>MAHHHHHHMPSERTFI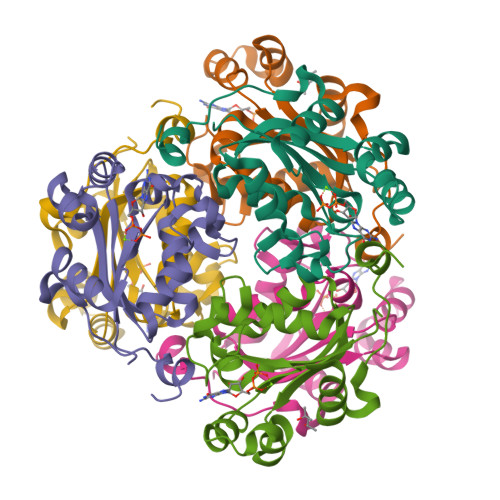AVKPDGVQRNLVGEIIKRFENKGYKLVGLKLLQPTEEQAKQHYIDLASKPFYSGLVSYFSSGPIVGMVWEGLGVVKGGRVLLGATNPADSLPGTIRGDFAVDVGRNVCHGSDSVESAKREIAFWFKAEELVSWTSHSVKQIYERA[3x]>GAMGKYVKVQDFYDQLGKYVLVAPGKFSGTVAATDLSTGWTMAWLAAWNYGDTCPIMHHMAAFPSPDPYKEFEFVVNTQGGKNLFIYGVPVTVEDPGEGMKIYRIKYDGTRMNLQRDAAEVSGLGLGVHVTITPEADGYAVGDGQKDICAEFDRETDMVRYAWAFDWDPNVKDLKRAWLDGGTMTIKRLKPTLPGGRYDLQGSKGNKIDWELVPGGELAIEDGKVSGDRPLHSVANDALVFDPRGKWAVASMRLPGVCVVFDRENQVPVAVLAGPKGTPSQFQLVKVDDDTWTVDIPEVISAGHQAGFSPDGQSFLFMNSLRQNNIMVWDSSNHDDPTTWEKKAVVESPDWRGAYP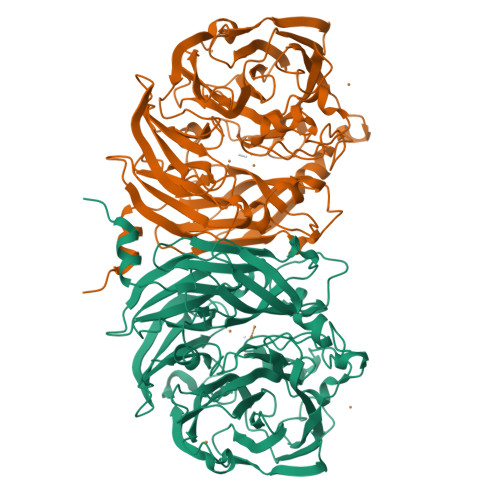NTFHMVFTPDAKKIYVTMWWPSPTPNGIAVIDAVNWEVLKEVDLGPDMHTLAITYDGKFVVGTLSGYQNTASAIVVMETETDEVLGFLPSPMGHHDNVIVPRTLEDLRISRSTTT[4x]>[2x]MNHKVHHHHHHMKANQVQPLNKYPVVFVHGFLGLVGDNAPALYPNYWGGNKFKVIEELRKQG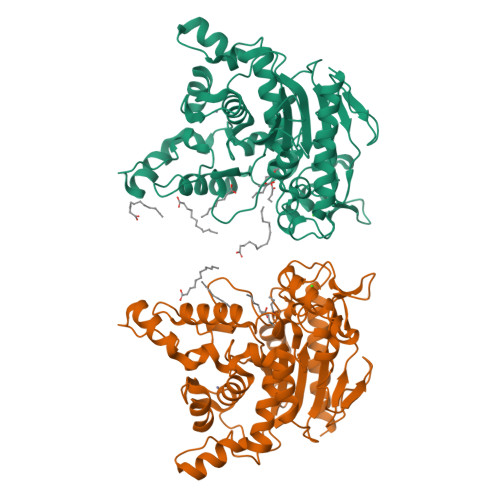YNVHQASVSAFGSNYDRAVQLYYYIKGGRVDYGAAHAAKYGHERYGKTYKGIMPNWEPGKKVHLVGHSMGGQTIRLMEEFLRNGNKEEIAYHQAHGGEISPLFTGGHNNMVASITTLATPHNGSQAADKFGNTEAVRKIMFALNRFMGNKYSNIDLGLTQWGFKQLPNESYIDYIKRVSKSKIWTSDDNAAYDLTLDGSAKLNNMTSMNPNITYTTYTGVSSHTGPLGYENPDLGTFFLMDTTSRIIGHDAREEWRKNDGVVPVISSLHPSNQPFVNVTNNEPATRRGIWQVKPILQGWDHVDFIGVDFLDFKRKGSELANFYIGIINDLLSVEATEGKGTQLKAS>[4x]HHHHHHMSKPDVSKLNRGNIVEFIGGIFDRRGDEEYLGEPVTMAEHMLQGATIAEQNGQPEEIIVGALLHDIGHFTSEFGMFSMDDTEDRYHEEAGAEVLEQFFPSVITDCVRYHVAAKRYL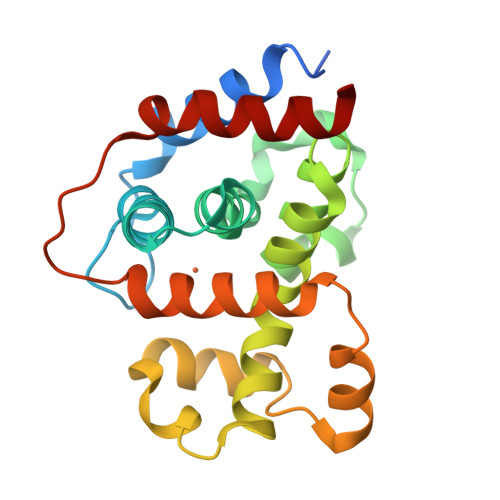CATKPEYFNRLSEASIHSLKLQGGPMDAEEVAEFEKNPNLKQIIAVRYLDEAGKRADMETPDYWHFAPMVQRMVDKHMGA> MMDMQVRKVRKPPACTQCRKRKIGCDRAKPICGNCVKYNKPDCFYPDGPGKMVAVPSASGMSTHGNGQGSNHFSQGNGVNQKNVMIQTQYPIMQTSIEAFNFSFNPSVDTAMQWTKAASYQNNNTNNNTAPRQNSSTVSSNVHGNTIVRSDSPDVPSMDQIREYNTRLQLV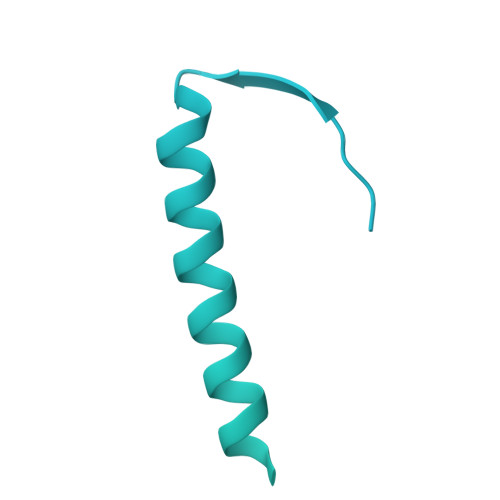NAQSFDYTDNPYSFNVGINQDSAVFDLMTSPFTQEEVLIKEIDFLKNKLLDLQSLQLKSLKEKSNLNADNTTANKINKTGENSKKGKVDGKRAGFDHQTSRTSQSSQKYFTALTITDVQSLVQVKPLKDTPNYLFTKNFIIFRDHYLFKFYNILHDICHINQFKVSPPNNKNHQQYMEVCKVNFPPKAIIIETLNSESLNNLNIEEFLPIFDKTLLLEFVHNSFPNGDTCPSFSTVDLPLSQLTKLGELTVLLLLLNDSMTLFNKQAINNHVSALMNNLRLIRSQITLINLEYYDQETIKFIAITKFYESLYMHDDHKSSLDEDLSCLLSFQIKDFKLFHFLKKMYYSRHSLLGQSSFMVPAAENLSPIPASIDTNDIPLIANDLKLLETQAKLINILQGVPFYLPVNLTKIESLLETLTMGVSNTVDLYFHDNEVRKEWKDTLNFINTIVYTNFFLFVQNESSLSMAVQHSSNNNKTSNSERCAKDLMKIISNMHIFYSITFNFIFPIKSIKSFSSGNNRFHSNGKEFLFANHFIEILQNFIAITFAIFQRCEVILYDEFYKNLSNEEINVQLLLIHDKILEILKKIEIIVSFLRDEMNSNGSFKSIKGFNKVLNLIKYMLRFSKKKQNFARNSDNNNVTDYSQSAKNKNVLLKFPVSELNRIYLKFKEISDFLMEREVVQRSIIIDKDLESDNLGITTANFNDFYDAFYN>MERLVKKVTSNLETELKFFKGRLVQELMQIVKNENGRIDHTSKNWQESASVLLNSQEKGAVSLAEVERAVSKMTQKLRDQKVSEEEVVNIESKLKFERASLEAKLFDDNEIKELINKRIKEDALRAIPFLGSDSESFMEKISPFVKLPDDSY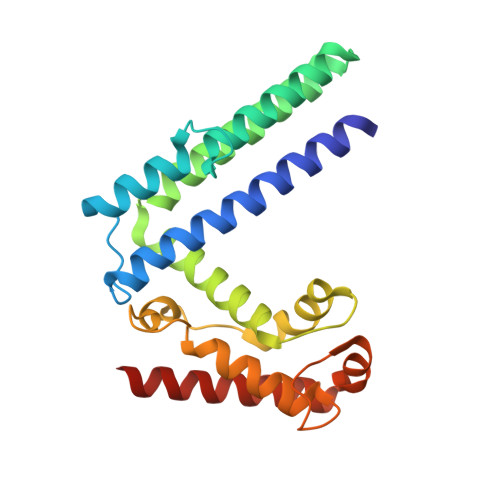SLLKANDKHHPFQNILYSNALKFFADSSDIGYLNDDSLKNLTPENLNAFEQAVAADIDKLMHHHHHH[6x]> MSNWVMQEENKQGNLTPLFEELLQQCPPGGQNKTAHMVSAYQLAQGNWMPTSCHVFMGTISARRTKTHPYEAYVKLRELVEEHKMKTLCPGSSLGKHNDWIIGKIKYQGNLRTKHMLNPGKVAEQLCREGHRHNVYNKTIGSVMTATGIRLEKLPVVRAQTDTTNFHQAIRDKIDKEENLQTPGLHKKLMEVFNALKRPELESSYDAVEWEELERGINRKGAAGFFERKNIGEILDSEKNKVEEIIDNLKKGRNIKYYETAIPKNEKRDVNDDWTAGDFVDEKKPRVIQYPEAKTRLAITKVMYKWVKQKPVVIPGYEGKTPLFQIFDKVKKEWDQFQNPVAVSFDTKAWDTQVTTKDLELIKDIQKYYFKKKWHKFIDTLTMHMTEVPVICADGEVYIRKGQRGSGQPDTSAGNSMLNVLTMVYAFCEATGVPYKSFDRVAKIHVCGDDGFLITERALGEKFASKGVQILYEAGKPQKITEGDKMKVAYQFDDIEFCSHTPIQVRWSDNTSSYMPGRNTTTILAKMATRLDSSGERGTIAYEKAVAFSFLLMYSWNPLIRRICLLVLSTELQVKPGKSTTYYYEGDPISAYKEVIGHNLFDLKRTSFEKLAKLNLSMSVLGAWTRHTSKRLLQDCVNMGVKEGNWLVNADRLVSSKTGNRYIPGEGHTLQGRHYEELVLARKGSSSHHHHHH

Compared to the RdRPs of other Flaviviridae representatives such as the NS5 of the Japanese encephalitis virus (JEV) and dengue virus (DENV) in the Flavivirus genus and the NS5B of the hepatitis C virus (HCV) of the Hepacivirus genus, the pestivirus NS5B contains a unique ∼90-residue N-terminal domain (NTD) that does not have notable sequence homology to any other viral or host proteins. The global conformation of our CSFV NS5B structures is consistent with the recently reported CSFV structure with an RMSD value of 0.9 Å (95% coverage) between the reported structure and our representative C-682 structure. These structures together reveal that the NTD adopts a globular α/β fold with an α-β-α-β-β-α pattern. The NTD interacts with the palm of the RdRP core intra-molecularly with a mixture of hydrophobic and hydrogen bonding interactions. Collectively, these biochemical data indicated that the RNA synthesis fidelity of CSFV NS5B is fine-tuned by its NTD through the intra-molecular interactions with the RdRP palm.

The structures of the C-682 and C-672 were solved at 2.1 and 2.3 Å resolution, respectively, in the same crystal form by molecular replacement using the structure of the WT as the search model. We hereinafter choose the highest-resolution C-682 structure as the primary structure for illustration with difference between structures discussed where necessary. In the structures of the WT and C-682, residues beyond 672 are disordered. The results indicated that residues 681–694 are not essential, as residue removal in this region did not apparently affect product level (compare lanes 7–9 to lane 6). The RdRP core of CSFV NS5B is structurally consistent with the BVDV structures, with an RMSD value of 1.5 Å (92% coverage) between the BVDV NS5B N438 duplication mutant structure and the CSFV C-682 structure. Different from the observations in the WT BVDV, full-length JEV, HCV and the recently reported CSFV RdRP structures that have a canonical fold optimal for NTP entry and binding, the CSFV NS5B ring finger bent toward the pinky finger, partially occupying the template RNA binding channel. Although this conformation is likely not compatible with de novo initiation, normal activity of the WT and C-682 observed in the polymerase assays suggests that the canonical conformation also exist in solution and may be in equilibrium with the observed bent conformation observed in the crystal structures. The aromatic ring of Y471 side chain is wrapped around by NTD resides 23–27 through hydrophobic interactions and its phenyl hydroxyl group forms a hydrogen bond with the carbonyl oxygen of C25 backbone, while the carboxyl group of the E472 side chain forms two hydrogen bonds with backbone amide nitrogen atoms of residues M56 and G57 and its two-carbon aliphatic side chain region interacts with P27 and V57 through hydrophobic interactions.> SNAMASLHIDDIPAAIKAVKQQLRQALPDYQQVFQAVEENIRQQVMEIRRNLAEGKNPVPQLHADDIINGKVTEEQKAQIKQRGCCAILGVFPQEKATAWNREIGDYLDR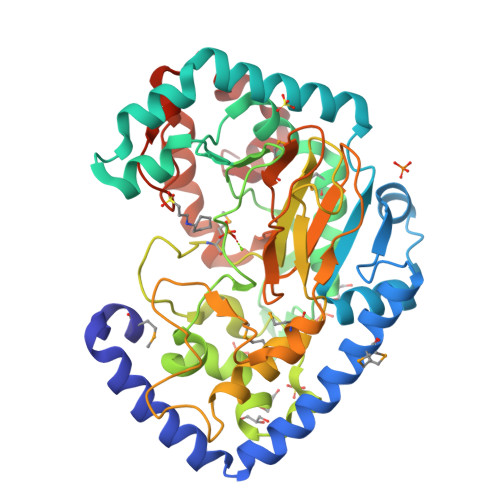NNFVERLKNAAEDNYFGTLAASKPQIYGIYWSTPQVEARQDKRMQAVQIFLNNLWQTESNGKQHFDANRVVTYADRTRRRPPKSSSLGLSPHVDGGSIERWLDENFRHVYRHVFSGQWQKYDPFAAEGRPEVREFPSPAVCSMFRTFQGWTALTPQRTHAGTLNVIPIANAMAYILLRALQDDVADDDLCGAAPGRALSASEQWHPLLMEAISPIPDLEAGDTVFWHCDVIHSVENEHNGEFDSNVMYIAAAPWCEKNAAYLPRQLASFIDGRSPPDFAADDFEVDFIGRATIKNLTEIGKQQLGITD> MKHFTAAVATVALSLALAGCSFNIKTDSAPTTSPTTTSPTTSTTTTSATTSAQAAGPN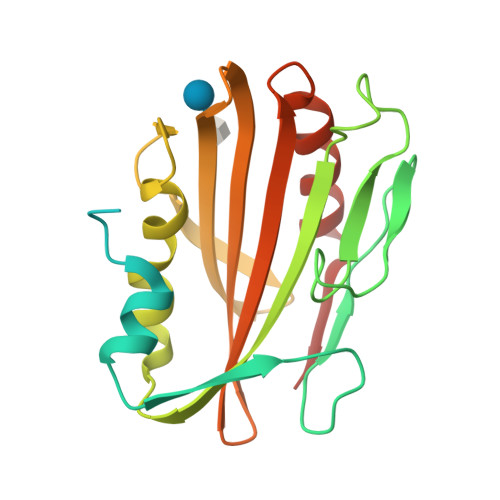YTIADYIRDNHIQETPVHHGDPGSPTIDLPVPDDWRLLPESSRAPYGGIVYTQPADPNDPPTIVAILSKLTGDIDPAKVLQFAPGELKNLPGFQGSGDGSAATLGGFSAWQLGGSYSKNGKLRTVAQKTVVIPSQGAVFVLQLNADALDDETMTLMDAANVIDEQTTITPHHHHHH>MKYVVVSGGVISGIGKGVLASSTGMLMKTLGLKVTSIKIDPYMNIDAGTMSPLEHGECFVLDDGGETDLDLGNYERYLGVTLTKDHNITTGKIYSHVIAKERKGDYLGKTVQIVPHLTNAIQDWIERVAKIPVDDTGMEPDVCIIELGGTVGDIESAPFVEALRQFQFKVGKENFALIHVSLVPVIHGEQKTKPTQAAIKGLRSLGLVPDMIACRCSETLDKPTIDKIAMFCHVGPEQVVNVHDVNSTYHVPLLLLEQKMIDYLHARLKLDEISLTEEEELLSKWKATTGNFDETVKIALVGKYTNLKDSYLSVIKALEHSSMKCRRKLDIKWVEATDLEPEAQESNKTKFHEAWNMVSTADGILIPGGFGVRGTEGMVLAARWARENHIPFLGVCLGLQIATIEFTRSVLGRKDSHSAEFYPDIDEKNHVVVFMMRLGLRPTFFQNETEWSQIKKLYGDVSEVHERHRHRYEINPKMVDELENNGLIFVGKDDTGKRCEILELKNHPYYIATQYHPEYTSKVLDPSKPFLGLVAASAGILQDVIEGKYDLEA[28x]

CTP synthase (CTPS) catalyzes the final, rate-limiting step of de novo CTP biosynthesis (Lieberman, 1956). Each CTPS monomer consists of a glutaminase domain and an amido-ligase domain connected by an alpha helical linker. Glutamine hydrolysis in the glutaminase domain produces ammonia which is transferred through a channel into the amido-ligase domain, where it is ligated to UTP to form CTP in an ATP-dependent process. Budding yeast have two CTPS isoforms, Ura7 and Ura8, which share 78 % identical residues.

We determined structures of CTPS filament bundles formed at pH 6.0 to better understand the mechanisms of lateral assembly. Reference-free two-dimensional averages of bundle segments from cryo-EM images of Ura7 and Ura8 were strikingly regular, suggesting ordered assembly contacts. This high degree of order allowed us to determine three-dimensional structures of both homologs in the presence of substrates or product using a single particle reconstruction approach by focused refinement of interacting pairs of filaments. As we found for the single filament structures, Ura8 reconstructions went to higher resolution (3.3 Å for substrates and 3.7 Å for product) than Ura7 (6.6 Å substrate and 7.0 Å product). The individual filaments that pack laterally in the bundles closely resemble the corresponding single filament structures. Ura7 formed very similar bundles in both ligand conditions, with adjacent filaments staggered relative to each other with a half-tetramer offset. Although at lower resolution, the Ura7 structures appear to make the same lateral contacts as substrate-bound Ura8. Yeast CTPS has a 7-residue insert (residues 273–279) in the linker region that mediates the bulk of the lateral interaction in both bundle types. Ura7 bundles in either ligand state are very similar, and at our resolution appear to maintain the same lateral contacts but with a slightly different helical twist. Regardless of nucleotide pools, bundles could therefore remain assembled to fulfill their role in the starvation response.> SNVPAELKYSKEHEWLRKEADGTYTVGITEHAQELLGDMVFVDLPE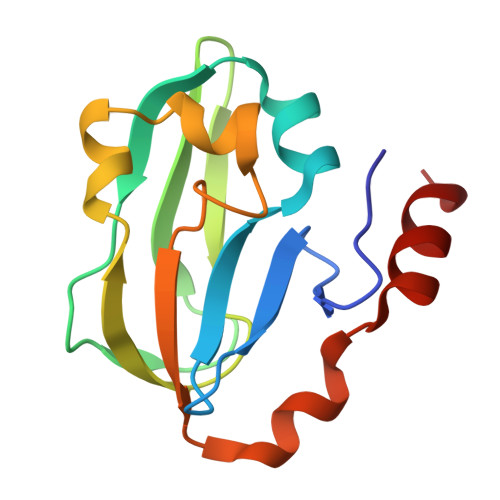VGATVSAGDDCAVAESVKAASDIYAPVSGEIVAVNDALSDSPELVNSEPYAGGWIFKIKASDESELESLLDATAYEALLEDE> MASMTGGQQMGRGSMSRDPLPFFPPLYLGGPEITTENCEREPIHIPGSIQPHGALLTADGHSGEVLQMSLNAATFLGQEPTVLRGQTLAALLPEQWPALQAALPPGCPDALQYRA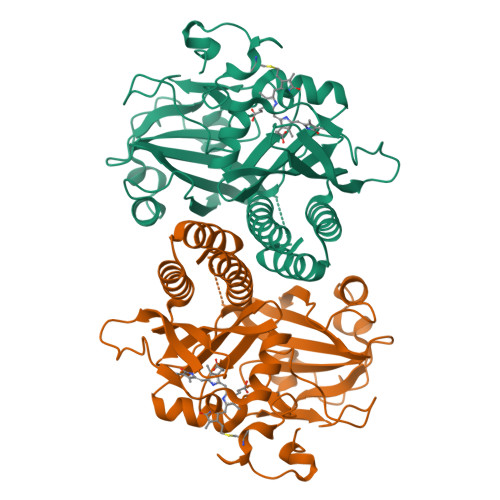TLDWPAAGHLSLTVHRVGELLILEFEPTEAWDSTGPHALRNAMFALESAPNLRALAEVATQTVRELTGFDRVMLYKFAPDATGEVIAEARREGLHAFLGHRFPASHIPAQARALYTRHLLRLTADTRAAAVPLDPVLNPQTNAPTPLGGAVLRATSPMHMQYLRNMGVGSSLSVSVVVGGQLWGLIACHHQTPYVLPPDLRTTLESLGRLLSLQVQVKEALEHHHHHH> SMNTDPLLPGFDYLTLHTSAARLRVAVKGSGPPLLLLHGYPQTHLAWHRIAPRLAEDYSVVLADLRGYGESRALDEEGADYSKAALARDQLETMGQLGFERFAVIGHDRGARVGYRLALDHPQAVAAFVSLTVVPILDNWAAVNKVFALNAYHWFLLAQPYDLPERLIGADPEHFLDYTLR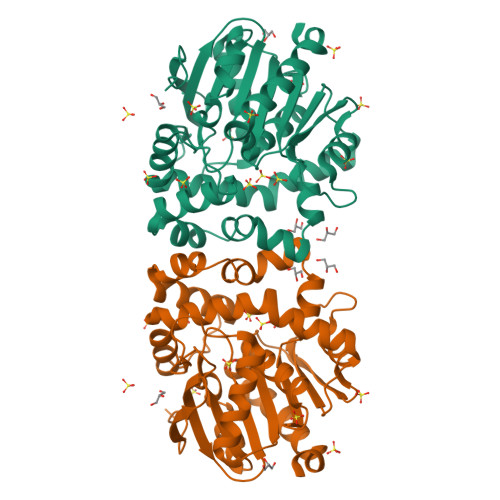RMAQGRDIYHPQALESYRRAFRDPAVRHAMCEDYRAAVGVDADADQADRDAGRRLQCPVQVLWQERPYAAGQHPLEIWKTWAGQVEGAAIGASHMLPEDAPDAVLEHLLGFLASHREALR> GYM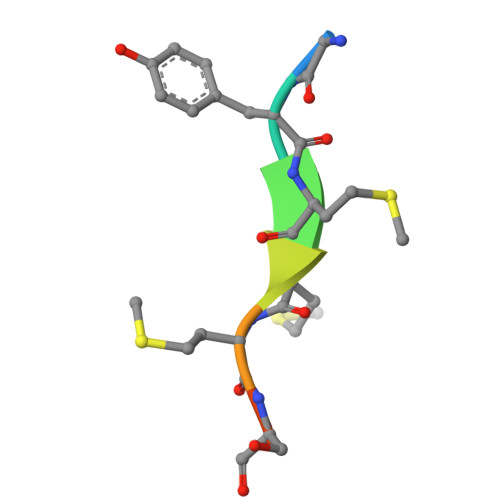MMSPS>GSHMN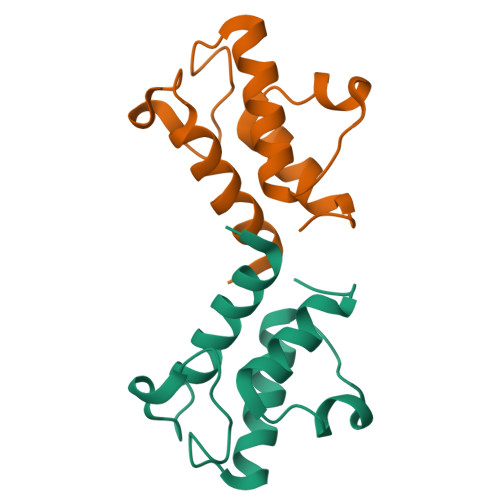DVLTRVLEVVKNFEKVDASKVTPESHFVKDLGLNALDVVEVVFAIEQEFILDIPDHDAEKIQSIPDAVEYIAQNPMAK[2x]> MTLEKFVDALPIPDTLKPVQQSKEKTYYEVTMEECTHQLHRDLPPTRLWGYNGLFPGPTIEVKRNENVYVKWMNNLPSTHFLPIDHT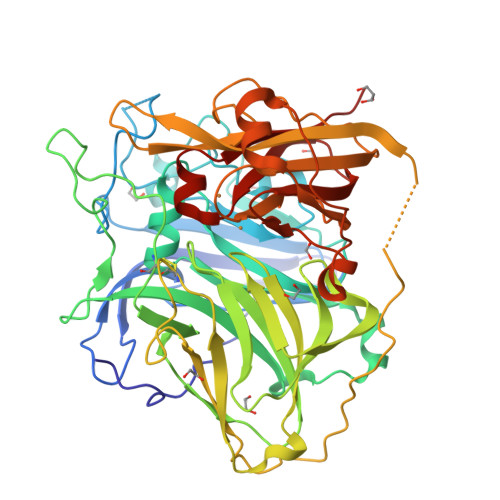IHHSDSQHEEPEVKTVVHLHGGVTPDDSDGYPEAWFSKDFEQTGPYFKREVYHYPNQQRGAILWYHDHAMALTRLNVYAGLVGAYIIHDPKEKRLKLPSDEYDVPLLITDRTINEDGSLFYPSAPENPSPSLPNPSIVPAFCGETILVNGKVWPYLEVEPRKYRFRVINASNTRTYNLSLDNGGDFIQIGSDGGLLPRSVKLNSFSLAPAERYDIIIDFTAYEGESIILANSAGCGGDVNPETDANIMQFRVTKPLAQKDESRKPKYLASYPSVQHERIQNIRTLKLAGTQDEYGRPVLLLNNKRWHDPVTETPKVGTTEIWSIINPTRGTHPIHLHLVSFRVLDRRPFDIARYQESGELSYTGPAVPPPPSEKGWKDTIQAHAGEVLRIAATFGPYSGRYVWCCHILEHEDYDMMRPMDITDPHK>GSHMDNQCTVQVRLELGHRAQLRKKPTTEGFTHDWMVFVRGPEQCDIQHFVEKVVFWLHDSFPKPRRVCKEPPYKVEESGYAGFIMPIEVHFKNKEEPRKVCFTYDLFLNLEGNPPVNPLNHLRCEKLTF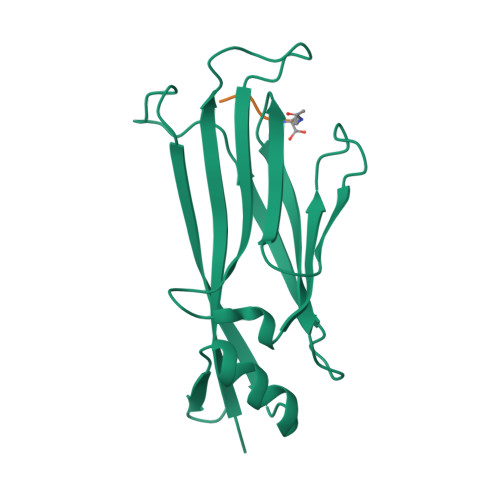NNPTTEFRYKLLRAGGVMVMPEGAHHHHHH[2x];>AARK[2x]>MTIVNRIRTDVVNVAKSFGAEYSEAVIDQIFQGFGEKFTNTGFAIRVQNKRNQKVDCNIRYGEAKENCLAWDIARESGLLSDQGHPVDTLIQEMFQAIPAIAYGADFDINYGLVKIWHLPKIVPVEEAFKIPSLPKSVNAHIDFFKKYHLDALCALTVDYRNKSTNLYFDAHHPEQRTTQFYKNILQSQQFEVPSDEVLEILVNCPEIAVTFNWSSPGIERMCFYTAFVNRETVPQHINPVLKKFAQEAPALLDNPGFLVGWSFGPDAKKGTYIKIDVDYHGLVV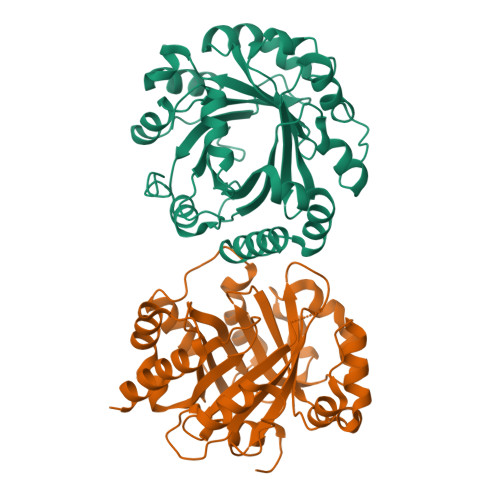PSFFHMHNLPLPIPEANSVFDLPSSDTEDKLNSIVMSKLAAALEHHHHHH[2x]>[18x]MNDNYQNNYVVGRGTVYFDRFQDGTNRKTGEMYFGNTPEFTINTDSETLDHYSSDHGMRVMDASVLLEASQGGTFTCDNINADNLALWFLGEVSNTTQTQQTDAKEVFNPIMRGRYYQLGTTDDNPTGVRGVTNFQMVKADASIAISVGSGDITSIVGATVVN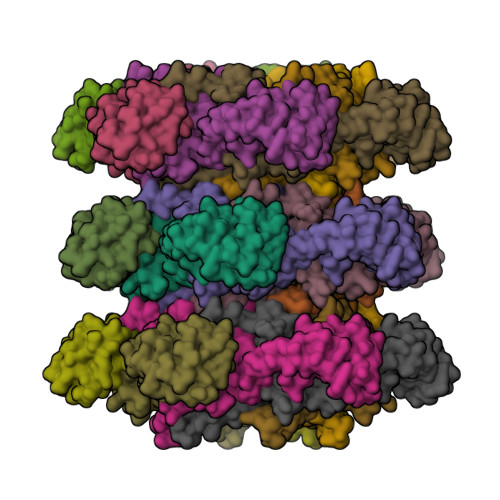PAGNYEIDLEAGRIYIEPDSTDLSGNVQIAVQYDVDAQKRTLVIGKSNMVYGALRMISDNPVGLNKNYYFPKVSIAPDGDYALKGDDWQVMSFTFKAMQLNNITQRVYIDIVEAAAAVDPTAQRTIEITPASTTATTGGAGVVCTVTVRDGTGTAVQGDAVTFTTVAGATVTPNSATTGASGTATTTVNRTAAGTATVTATLANGKAATTGTITFSAP>SVAADLPALPGGPAGGTGELAKYGLPGVAQLRSRESYVLSYDPRTRGALWVLEQLRPERLRGDGDRSACDFREDDSVHAYHRATNADYRGSGFDRGALAAAANHRWSQRAMD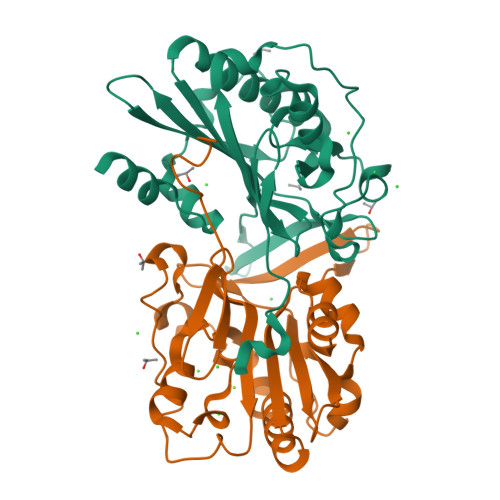DTFYLSNVAPQVPHLNQNAWNNLERYSRSLTRTYQNVYVCTGPLFLPRTEADGKSYVKYQVIGKNHVAVPTHFFKVLILEAAGGQIELRSYVMPNAPVDETIPLERFLVPIESIERASGLLFVPNILARAGNLKAITAGSK[2x]> GPMAQQKVVLKVPTMTDEKTKQKAIEAVADIYGIDSIAADLKDNKMTIIGDMDTVEIAKKLRKIGKIDIVSVGPA;> GHMAAPARFCVYYD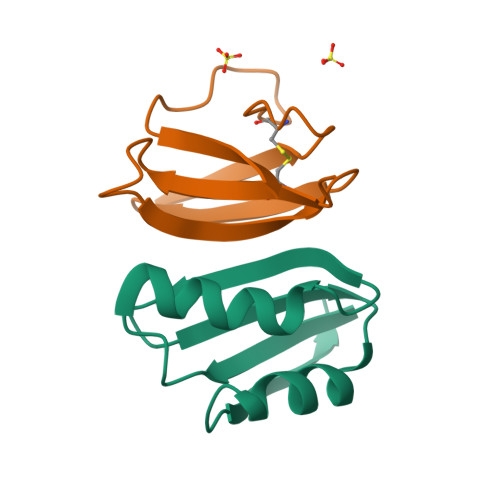GHLPATRVLLMYVRIGTTATITARGHEFEVEAKDQNCKVILTNGKQAPDWLAAEPY>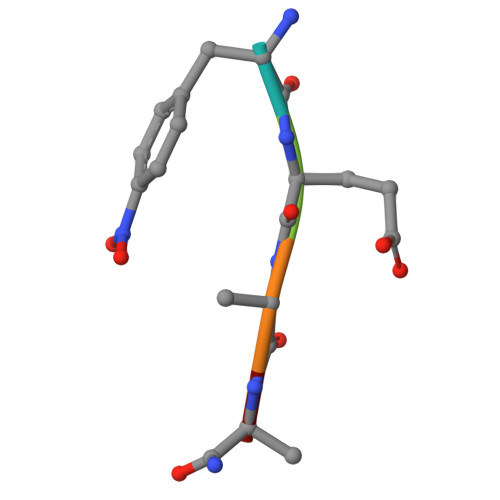 FEALS> GSPGISGGGGGSHIEGYECQPIFLNVLEAIEPGVVCAGHDNNQPDSFAALLSSLNELGERQLVHVVKWAKALPGFRN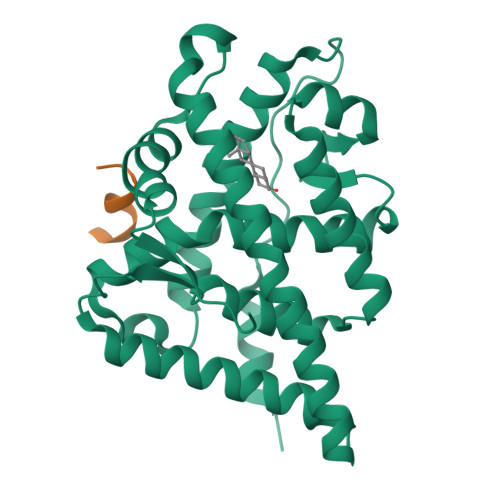LHVDDQMAVIQYSWMGLMVFAMGWRSFTNVNSRMLYFAPDLVFNEYRMHKSRMYSQCVRMRHLSQEFGWLQITPQEFLCMKALLLFSIIPVDGLKNQKFFDELRMNYIKELDRIIACKRKNPTSCSRRFYQLTKLLDSVQPIARELHQFTFDLLIKSHMVSVDFPEMMAEIISVQVPKILSGKVKPIYFHTQ;> SSKFAALWDPPKLSRSGSGK> MSLVNGMVESLNNTKSETEIGIGGYRLFARVRETVNYRNIVPTDTLEDGSSSTDDIINEPITVSIEGVVSNLFVEERQYPQLVSRDFSAVGEITALLPAKSQQQIQRISQIDSQIRDAVLAAERAERLAGKPYEFFGNSGNSAKTEQEKFIDFMEALYFSRRPTEVSVNFRDYKNMALVSFIPVRDN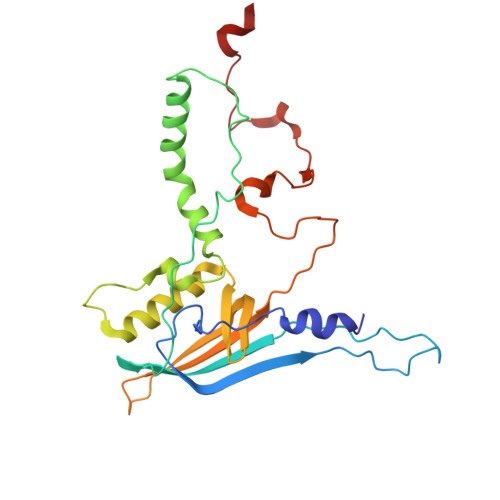NTKDTRFTADFQQINYSTLVYTPVSSPSKSVSGKVSDASNKGGQNPESNETGERSLLSSLVGG>GSAMGSASTSGNPFQANVEMKTFMERFNLTHHHQSGIYVDLGQDKEVDGTLYREPAGLCPIWGKHIELQQPDRPPYRNNFLEDVPTEKEYKQSGNPLPGGFNLNFVTPSGQRISPFPMELLEKNSNIKASTDLGRCAEFAFKTVAMDKNNKATKYRYPFVYDSKKRLCHILAVSMQLMEGKKYCSVKGEPPDLTWYCFKPRKSVTENHHLIYGSAYVGENPDAFISKCPNQALRGYRFGVWKKGRCLDYTELTDT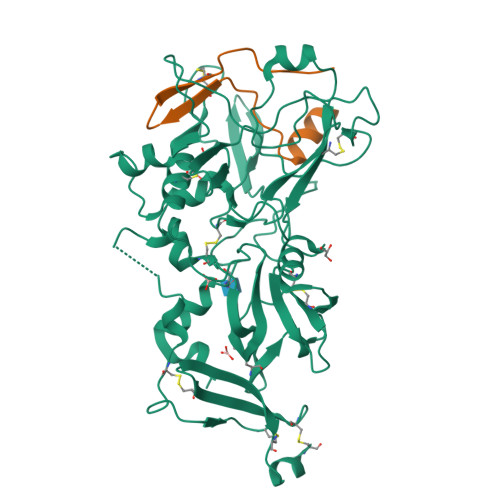VIERVESKAQCWVKTFENDGVASDQPHTYPLTSQASWNDWWPLHQSDQPHSGGVGRNYGFYYVDTTGEGKCALSDQVPDCLVSDSAAVSYTAAGSLSEETPNFIIPSNPSVTPPTPETALQCTADKFPDSFGACDVQACKRQKTSCVGGQIQSTSVDCTADEQNECGSNTAAALVPR[2x];>DIVQHMEDIGGAPPVSCVTNEILGVTCAPQAIAKATT[2x]> NTVTEDTPATEQAVETPQPTAVSEEAPSSSKETKIPQTPGDAEETVADDANDLAPQAPAKTADTPATSKATIRDLNDPSQVKTLQEKAGKGAGTVVAVIDAGFDKNHEAWRLTDKTKARYQSKEDLEKAKKEHGITYGEWVNDKVAYYHDYSKDGKTAVDQEHGTHVSGILSGNAPSETKEPYRLEGAMPEAQLLLMRVEIVNGLADYARNYAQAIRDAVNLGAKVINMSFGNAALAYANLPDETKKAFDYAKSKGVSIVTSAGNDSSFGGKTRLPLADHPDYGVVGTPAAADSTLTVASYSPDKQLTETATVKTDDHQAKEMPVLSTNRFEPNKAYDYAYANRGMKEDDFKDVKGKIALIERGDIDFKDKIANAKKAGAVGVLIYDNQDKGFPIELPNVDQMPAAFISRKDGLLLKDNSKKTITFNATPKVLPTASDTKLSRFSSWGLTADGNIKPDIAAPGQDILSSVANNKYAKLSGTAMSAPLVAGIMGLLQKQYETQYPDMTPSERLDLAKKVLMSSATALYDEDEKAYFSPRQQGAGAVDAKKASAATMYVTDKDNTSSKVHLNNVSDKFEVTVTVHNKSDKPQELYYQATVQTDKVDGKHFALAPKALYETSWQKITIPANSSKQVTVPIDASRFSKDLLAQMKNGYFLEGFVRFKQDPKKEELMSIPYIGFRGDFGNLSALEKPIYDSKDGSSYYHEANSDAKDQLDGDGLQFYALKNNFTALTTESNPWTIIKAVKEGVENIEDIESSEITETIFAGTFAKQDDDSHYYIHRHANGKPYAAISPNGDGNRDYVQFQGTFLRNAKNLVAEVLDKEGNVVWTSEVTEQVVKNYNNDLASTLGSTRFEKTRWDGKDKDGKVVVNGTYTYRVRYTPISSGAKEQHTDFDVIVDNTTPEVATSATFSTEDRRLTLASKPKTSQPIYRERIAYTYMDEDLPTTEYISPNEDGTFTLPEEAETMEGGTVPLKMSDFTYVVEDMAGNITYTPVTKLLEG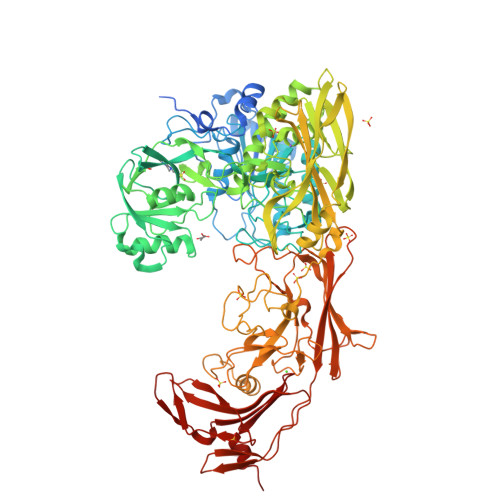HS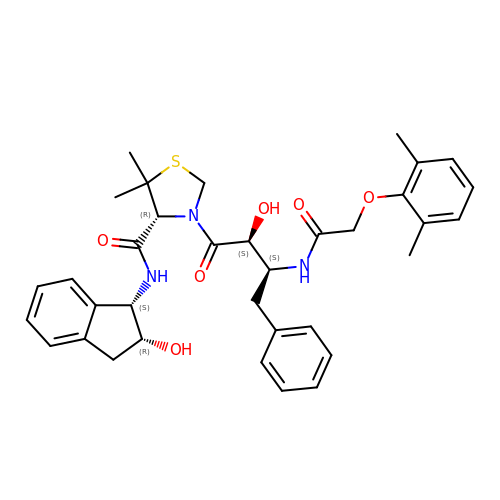(4R)-3-[(2S,3S)-3-{[(2,6-dimethylphenoxy)acetyl]amino}-2-hydroxy-4-phenylbutanoyl]-N-[(1S,2R)-2-hydroxy-2,3-dihydro-1H-inden-1-yl]-5,5-dimethyl-1,3-thiazolidine-4-carboxamide | C35 H41 N3 O6 S | KKTYZYHUPKXLPL-RIQJEONASA-N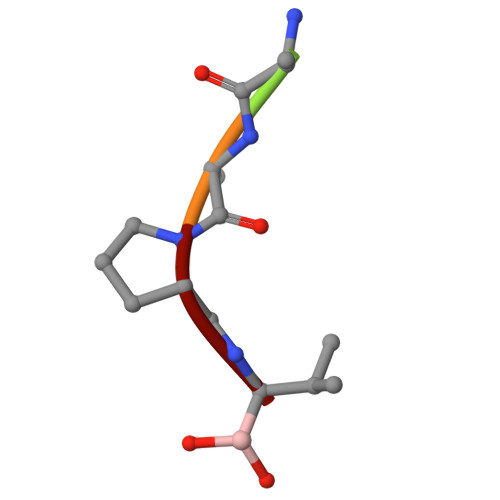> XAAPV We have therefore investigated the functional behaviors of an interaction network hypothesized from available structural data in the Escherichia coli alkaline phosphatase (AP) active site. Nevertheless, these residues are part of an extensive hydrogen-bonded and Mg2+-coordinating network that also involves D101, D153, K328, the Mg2+ ion liganded by E322, and two water molecules. We observed three overlapping functional units, D101/R166/D153, D153/Mg2+/K328, and D101/Mg2+.

The simplest model to account for these effects is that each aspartate residue helps to position the arginine side chain for interaction with the non-bridging phosphoryl oxygen atoms. To further explore the effects of the aspartate residues on the R166 functional unit, we solved the crystal structure of D101A/D153A AP. In one subunit of the AP homodimer, the guanidinium group is flipped away from the active site and adopts a catalytically unproductive conformation that is similar to the conformation observed in one structure of D153G, but more displaced than in the other structure of D153G and D101S AP. In the other monomer, R166 was observed to populate two rotameric positions, one of which is similarly flipped away from the active site while the other is pointed towards the active site. Although this structure lacks a bound Mg2+ ion in the active site, the functional and structural data presented above suggest that this loss will not influence the position of R166. In both active sites of D101A/D153A AP, the bound Pi is not well positioned, populating multiple conformations that are each distinct from its position in WT AP, which likely closely mimics the reactive phosphoryl conformation. These structural comparisons provide evidence that the aspartate residues that flank R166 help to correctly position the reactive phosphoryl group and provide a self-consistent picture of the functional effects of the D101/R166/D153 functional unit. The aspartate residues of the D101/R166/D153 unit make nearly independent contributions to the catalytic function of the central arginine residue; D153 and K328 (and presumably their associated water molecules) act cooperatively with the Mg2+ ion and increase its contribution to catalysis; and the Mg2+ ion and D101 are energetically anti-cooperative and apparently constitute a redundant functional unit.

>[2x]NRAAQGDITAPGGARRLTGDQTAALRDSLSDKPAKNIILLIGDGMGDSEITAARNYAEGAGGFFKGIDALPLTGQYTHYALNKKTGKPDYVTASAASATAWSTGVKTYNGALGVDIHEKDHPTILEMAKAAGLATGNVSTAELQAATPAALVAHVTSRKCYGPSATSEKCPGNALEKGGKGSITEQLLNARADVTLGGGAKTFAETATAGEWQGKTLREQAQARGYQLVSDAASLNSVTEANQQKPLLGLFADGNMPVRWLGPKATYHGNIDKPAVTCTPNPQRNDSVPTLAQMTDKAIELLSKNEKGFFLQVEGASIDKQDHAANPCGQIGETVDLDEAVQRALEFAKKEGNTLVIVTADHAHASQIVAPDTKAPGLTQALNTKDGAVMVMSYGNSEEDSQEHTGSQLRIAAYGPHAANVVGLTDQTDLFYTMKAALGLKSA>[2x]MKSTPFFYPEAIVLAYLYDNEGIATYDLYKKVNAEFPMST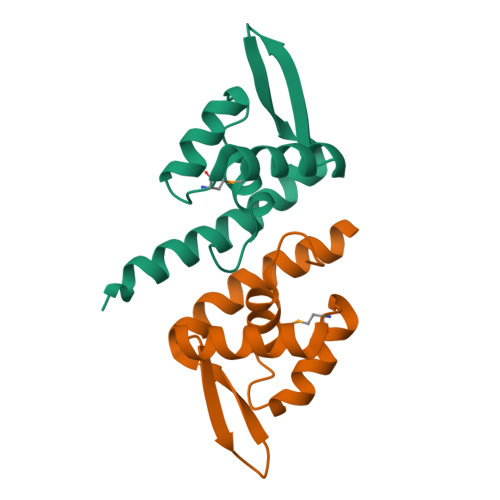ATFYDAKKFLIQEGFVKERQERGEKRLYLTEKGKLFAISLKTAIETYKQIKKRHHHHHH>MKMDKKTIVWFRRDLRIEDNPALAAAAHEGSVFPVFIWCPEEEGQFYPGRASRWWMKQSLAHLSQS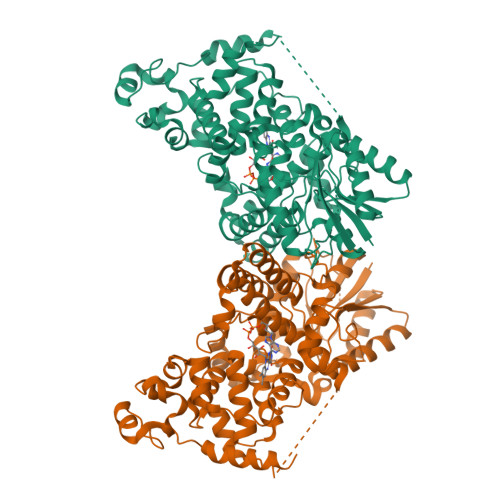LKALGSDLTLIQTHNTISAILDCIRVTGPTKVVFNHLYDPVSLVRDHTVKEKLVERGISVQSYNGDLLYEPWEIYCEKGKPFTSFNSYWKKCLDMSIESVMLPPPWRLMPITAAAEAIWACSIEELGLENEAEKPSNALLTRAWSPGWSNADKLLNEFIEKQLIDYAKNSKKVVGNSTSLLSPYLHFGEISVRHVFQCARMKQIIWARDKNSEGEESADLFLRGIGLREYSRYICFNFPFTHEQSLLSHLRFFPWDADVDKFKAWRQGRTGYPLVDAGMRELWATGWMHNRIRVIVSSFGVKFLLLPWKWGMKYFWDTLLDADLECDILGWQYISGSIPDGHELDRLDNPALQGAKYDPEGEYIRQWLPELARLPTEWIHHPWDAPLTVLKASGVELGTNYAKPIVDIDTARELLAKAISRTREAQIMIGAAPDEIVADSFEALGANTIKEPGLCPSVSSNDQQVPSVVRYNGSKRVKPEEEEERDMKKSRGFDERELFSTAESSSSSSVFFVSQSCSLASEGKNLEGIQDSSDQITTSLGKNGCK[2x]>AYTTFSQTKNDQLKEPMFFGQPVNVARYDQQKYDIFEKLIEKQLSFFWRPEEVDVSRDRIDYQALPEHEKHIFISNLKYQTLLDSIQGRSPNVALLPLISIPELETWVETWAFSETIHSRSYTHIIRNIVNDPSVVFDDIVTNEQIQKRAEGISSYYDELIEMTSYWHLLGEGTHTVNGKTVTV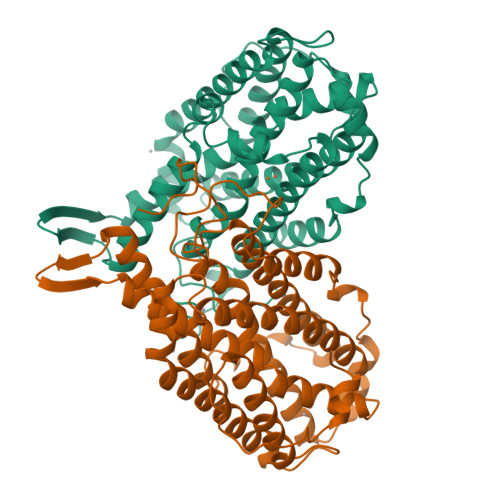SLRELKKKLYLCLMSVNALEAIRFYVAFACSFAFAERELMEGNAKIIRLIARDEALHLTGTQHMLNLLRSGADDPEMAEIAEECKQECYDLFVQAAQQEKDWADYLFRDGSMIGLNKDILCQYVEYITNIRMQAVGLDLPFQTRSNPIPWINTWLV[2x]>[10x]NLLRKNVDTLTPDEILNLQVSLRAMQDDEGASGYQAISAYHGEPADCKAADGSTIVCCLHGMPTFPMWHRLYLVQFEQALVAHGSTLGIPYWDWTKPMTQLPELVQHPLFIDPTGKKAKKNVFYSGEIKFENKVTARAVDARLYQASQEGQKNFLLEGVLNALEQEDFCHFEVQLEVAHNPIHYLVGGRFTHSMSSLEYTSYDPLFFLHHSNVERHFALWQALQKHRGLPTRPNCGLNLFHSPMEPFGRDTNPFAITKDNSKASSLFDYEHLGYAFDDLSLNGMTIEELEALLKQRRSGARAFANFRLGGIKTSANVRIKLCIPTEDKRQSDNCDNDAGQFFILGGTNEMPWNFAFPYLHEITDTVLSLGLALDSNYYVTAEVTAINGTLMPTQTIPRPIVTYIPPQGFKDVNMVNMDTSSLRFRKDISSLTTEEEYELRVAMERFMSDKSINGYQALAEFHGLPAKCPRPDALNRVACCIHGMATFPHWHRLVVMQFENALFTRGSPIGVPYWDWTKPFTALPSLLADETYVDPYTKETKPNPFFKAPIEFLKAGVHTSRQIDERLFKQPSKGDHGFLYDGLSLAFEQDDFCDFEVQFEVTHNSIHAWTGGSEPYSMSSLHYTSFDPMFWLHHSQVDRLWAIWQALQIQRGKPYKTYCANSEVYRPMKPFAFKSPLNNDEKTREHSVPTDVYDYQAELAYTYDTLFFGGLSIRELQRYVEEAKSKDRVFAGFLLMGIQTSANVDLFVVAGGNEFFVGSIAVLGGSKEMTWRFDRVYKHEITDALGALGVDMFAEYTLRVDIKD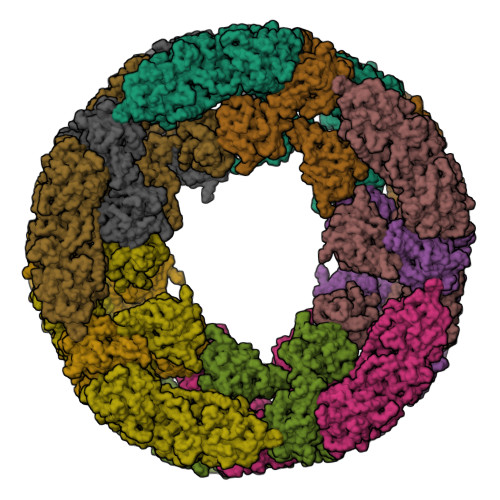VNGTALPPTAIPPPIVIFVPGIADANVKFDEQHRSRKNVDSMTVSEMNALRTAMAAFAADKEVTGYQQVAAFHGSTQWCPSPDAAQKYACCHHGMATFPHWHRLIALNFENGLRRNGWSGGLPYWDWTRPIDALPALVLEAEYTDANGEAKPNPFFSGAIDSIGASTSRAPTEALYEKPDFGKYTHLANEIISALEQEDFCDFEVQYEIAHNHIHALVGGTEAVSMASLEYSAFDPIFMLHHSNVDRIWATWQALQKFRGKAYNSANCAIEILRKPMSPFSLASDINPDAMTREYSVPFDVFNYKKNFHYEYDTLELNGLSIXQLSREINRRKAKNRVXVTFMLEGLKKSLLVEYFIAADGTDQKMKAGEFYVLGSENEMPWKFDRPYKSDITYVMDAMKLHYTDKYHVELRITDMTGAEVTDLKLVTSVIYEPGIGNFGEGRRWISPITSASRIRKNLLDFEDGEMESLRNAFKQMADEGRYEEIASFHGVPAQCPSEDGTMVHTCCLHGMPVFPHWHRLYVSLVEDELLARGSGVAVPYWDWVEPFDELPRLINEATFYNSRTLQIEPNPFFKGKISFENAETDRDTQPELFGNRYLYDHTLFVFEQTDFCEFEVHYEVLHNTIHSWLGGRDVHSMSSLDYAAYDPVFFLHHSNVDRLWAIWQELQRYRKLSYNEANCALPLMNQPMRPFSNSTANNDRLTFTNSRPNDVFDYQNVLHYKYDTLNFAGLSIPQLERILQKNQGRDRIFAGFLLHGIKASADVRIYICVPTGIGEENCGNYAGIFSVLGGETEMPWQFDRLFRYEITDELKKLGLNQNSHFRVEMELTAVNGSKITQKIFPNPTIIFVPSDVEFEEDTWRDVVTSANRIRRNLKDLSKEDMFSLRAAFKRMTDDGRYEEIAAFHGLPAQCPNADGSNIHTCCLHGMPTFPHWHRLYLSLVENELLARGSDVAVPYWDWIEPFDSLPGLISDETYKHPKTNEDIENPFHHGKISFADAVTVRKPRDQLFNNRYLYEHALFAFEHTDFCDFEVHFEVLHNSIHSWIGGPNPHSMSSLDFAAYDPIFFLHHSTVDRLWAIWQDLQRYRKLDYNVANCALNLLNDPMRPFNNKTANQDHLTFTNSRPNDVFDYQNSLNYKFDSLSFSGLSIPRLDDLLESRQSHDRVFAGFWLSGIKASADVNIHICVPIGVEHEDCDNYAGTFAVLGGETEMPWAFDRLFRYEISDEMKKLQLTEDSKFRLTTNIIASNGSKVSNDIFPTPTVIFVPKKERTEQVSTTKSVRGNLVRKNVDRLSLQEINSLIHALKRMQKDRSSDGFETIASFHALPPLCPNPTAKHRHACCLHGMATFPQWHRLYVVQFEHSLNRHGAIVGVPYWDWTYPMTEVPGLLTSEKYTDPFTGIETFNPFNHGHISFISPETMTTREVSEHLFEQPALGKQTWLFNNIILALEQTDYCDFEVQFEIVHNSIHSWLGGKELYSLNHLHYAAYDPAFFLHHSNVDRLWVVWQELQKFRGLPAYESNCAIELMSQPLKPFSFGAPYNLNPVTTKYSKPSDVFNYKQNFHYEYDMLEMNGMSIAQLESYIRQERQKDRVFAGFLLEGFGSSAYATFQVCPDVGDCYEGSHFSVLGGSTEMPWAFDRLYKMEITDILQAMDLKFDSHFTIKTKIVAHNGTELPESLLPEATIVRIPPSAQNLEVAIPLNRIRRNINSLESRDVQNLMSALKRLKEDESDFGFQTIAGYHGSLMCPTPEAPEYACCLHGMPTFMHWHRVYLLHFEESMRRHGASVAVPYWDWTMPSDNLPSLLGDADYYDAWTDSVIENPFLRGHIKYEDTYTVREIQPELFALAEGQKESTLFKDVMLMFEQEDYCDFEVQAEVIHNSIHYLIGGHQKYAMSSLMFSSFDPIFYVHHSMVDRLWAIWQELQKHRKLPHDKAYCALDQMAFPMKPFIWESNPNPTTRAVSTPSKLFDYKSLGYDYDHLNFHGMSIGQLEALIQKQKKADRVFAGFLLHGIKISADVHLKICIEADCQEAGVIFVLGGETEMPWHFDRNYKMDITDVLKKRNIPPEALFEHDSKIRLEVEIKSVDGAVLDPNSLPKPSLIYAPAKGLIIQQVGEYDAGSMVRKNVNSLTPSEIENLRNALAAVQADKTDAGYQKIASFHGMPLSCQYPDGTAFACCQHGMVTFPHWHRLYMKQMEDALKAKGAKIGIPYWDWTTAFHSLPILVTEPKNNPFHHGYIDVADTKTTRDPRPQLFDDPEQGDQSFFYRQIAFALEQRDFCDFEIQFEMGHNAIHSWVGGPSPYGMSTLHYTSYDPLFYVHHSNTDRIWAIWQALQKYRGLPYNSANCEINKLKKPMMPFSSEDNPNEVTKAHSTGYKSFDYQQLNYEYDNLNFHGMTIPQLEVHLKKIQEKDRVFAGFLLRAIGQSADVNFDVCRKDGECTFGGTFCVLGGDYEMPWAFDRLFLYDISKSLVHLRLDAHDDFDIKVTIMGIDGKSLPPNLLPSPTILFKPGTGKI>MHHHHHHSSGRENLYFQGHMDRLITLVVSYSIAFSIFALATMAVVYGKWLYYFEIDFLNIPDLADMTKDEIKRNYDVLITYLSPFYDGALHLPTLDMSTNGRIHFVDVKNILVKIQYVMYATIMIAVIGGIYLLKKKNEKFLLHGSILT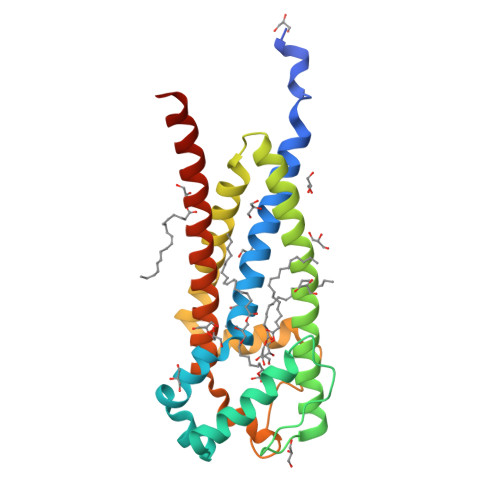IIFPIALMLPIAINFEKSFVLFHKLLFSNDYWVFDPEKDPIILMLPEEFFMHAACAILLFILGGSILCYSLYRYLVKKKRMSQKKFSA[2x]>SMMELRVGNRYRLGRKIGSGSFGDIYLGTDIAAGEEVAIKLECVKTKHPQLHIESKIYKMMQGGVGIPTIRWCGAEGDYNVMVMELLGPSLEDLFNFCSRKFSLKTVLLLADQMISRIEYIHSKNFIHRDVKPDNFLMGLGKKGNLVYIIDFGLAKKYRDARTHQHIPYRENKNLTGTARYASINTHLGIEQSRRDDLESLGYVLMYFNLGSLPWQGLKAATKRQKYERISEKKMSTPIEVLCKGYPSEFATYLNFCRSLRFDDKPDYSY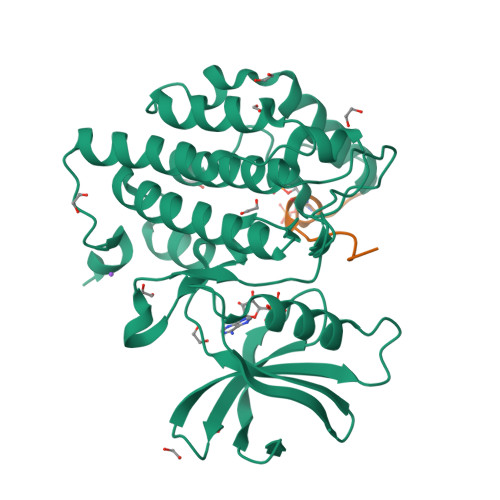LRQLFRNLFHRQGFSYDYVFDWNMLK[2x];>YTPSSASTVSVGSSET[2x]> GLTYCTHASGFSFNPQTADAGTSMNVVTEQIYNKLFDIKNHSATLTPMLAQSYSISADGKEILLNLRHGVKFHQTPWFTPTRDFNAEDVVFSINRVLGHNTYLPTLAEANVTYSNPQYKVFHEQARKVRFPYFDSIKLNEKIKSVTALSPYQVKIELFAPDSSILSHLASQYAIIFSQEYAYQLSADDNLAQLDTHPVGTGPYQVKDYVYNQYVRLVRNENYWKKEAKIEHIIVDLSTDRSGRLVKFFNNECQIASYPEVSQIGLLKNDDKHYYMQSTDGMNLAYLAFNFDKPLMRDHEIRAAISQSLNRARIIHSIYHNTATVANNIIPEVSWASTVNTPEFEFDYHPKIAKNKLADKNLLLNLWVINEEQVYNPAPFKMAEMIKWDLAQAGVKVKVRAVTRPFLTAQLRNQSENYDLILSGWLAGNLDPDGFMRPILSCGTKNELTNLSNWCNEEFDQFMDRAITTSHLSSRAKAYNEAQELVLRELPIIPIANVKRILVANSRVKGVKMTPFGSLDFSTLYFI

Important for NTHi survival, colonization and persistence in vivo is the Sap (sensitivity to antimicrobial peptides) ABC transporter system. An essential system for NTHi survival and persistence in vivo is the Sap (sensitivity to antimicrobial peptides) transporter. This multi-component system uses a periplasmic protein (SapA) to bind and deliver substrates to the heterodimeric inner membrane-associated Sap permease (SapBC). The Sap ABC transporter is completed by two membrane-associated nucleotide-binding proteins (SapD & SapF) that hydrolyze ATP to provide energy for substrate transport across the bacterial inner membrane. The structure confirmed the classification of SapA into the Substrate Binding Protein (SBP) superfamily, as was predicted from sequence analysis.

Here, the crystal structure of SapA, the periplasmic component of Sap, in a closed, ligand bound conformation, is presented. Crystals were nevertheless obtained and the structure of the 60 kDa SapA protein was solved to a resolution of 2.6 Å. In SapAclosed, the lobes enclose a cavity with two narrow openings to the protein surface. Difference electron density (Fo—Fc) became apparent within this cavity during the later stages of refinement. Since the location of the SapAclosed cavity approximately coincides with the ligand binding cavities of other SBPs, we inferred that this density might represent an endogenous ligand likely derived from the cell lysate. The presence of an endogenous ligand rationalizes the observed closed conformation of SapAclosed. The SapA cavity volume is even smaller again at approximately 400 Å3, which implies that SapA can only bind a small ligand such as a single amino acid or dipeptide. SapA co-crystallized with a strand of endogenously acquired RNA coordinated on the opposite face to the binding cleft. The RNA crystallized as a double helix with parameters consistent for standard A-form dsRNA, with a radius of ~12 Å and pitch of 31 Å with 11 bp per turn and a rise per bp of 2.8 Å (31 Å/11 bp). Specifically, the guanidino group of Arg 101 forms a hydrogen bond with the ribose 2’ hydroxyl and the 3’oxygen.> MASPIESARIGEVKRETKETNVSVKINLDGHGVSDSSTGIPFLDHMLDQLASHGLFDVHVRATGDTHIDDHHTNEDVALAIGTALLKALGERKGINRFGDFTAPLDEALIHVSLDLSGRPYLGYNLEIPTQRVGTYDTQLVEHFFQSLVNTSGMTLHIRQLAGKNSHHIIEATFKAFARALRQ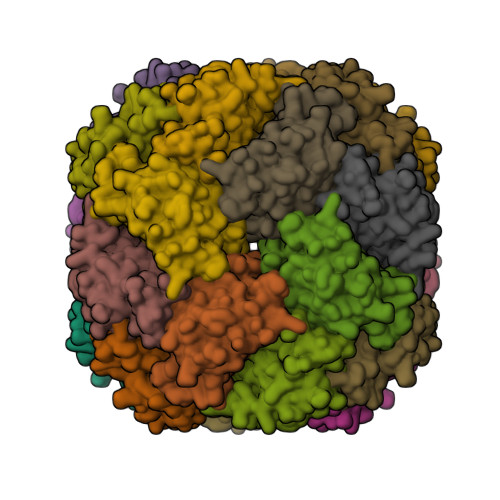ATESDPRRGGTIPSSKGVLSRS>MNHKVHHHHHHIEGRHMSPYAAPVRDHAGNLRDYLLAAGKATPDKPAIVEPAEDGGLRFVSYRQLEAQADAYAAELDALGLDVGDRVVLESPATADAVAAFLACFSLGLPFIPTIPETPVQRLRTIIGMAAPALFLQAADGSREGLPPGLGMARFGPKGVTTEQLPAPRVRRRRQVVETDPAYLIFTSGTTGRPKGVVMSHRANIAFHRGIRAHGLIGPDDRVAVTSPFSFDFCLGGIALTLASGATAVPVPRDRLDFPRRFLAFLHEAAITQVHGVPSLWRPLIRHEPDLVAGLDPLRSILFSGEDFPLGDLRELQGLLPGRRIFNLYGATESMAASVTDVPDPLPADLERLTIGYAHHGAEMDVYDAEGAPVGEPGVVGEIYLRSPALFSGYWADPEATRAALVPDPLLPESGQVVFRTGDLAYRDADGRLYFCGRIDSQVQIRGNRVELGEVERRLREFPGVSGAVALVAPAGEGEPELSAFLTMRPGAPAPKLVPLRAFCAETLPEYMAPRSLTVLAELPVTTNGKIDKDAL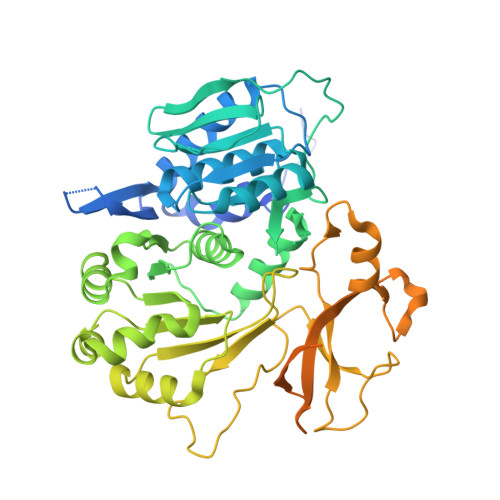LRARTAR[4x]> ARLGRQALLFPLCLVLYEFSTYIGNDMIQPGMLAVVEQYQAGIDWVPTSMTAYLAGGMFLQWLLGPLSDRIGRRPVMLAGVVWFIVTCLAILLAQNIEQFTLLRFLQGISLCFIGAVGYAAIQESFEEAVCIKITALMANVALIAPLLGPLVGAAWIHVLPWEGMFVLFAALAAISFFGLQRAMPETATRIGEKLSLKELGRDYKLVLKNGRFVAGALALGFVSLPLLAWTAQSPIIIITGEQLSSYEYGLLQVPIFGALIAGNLLLARLTSRRTVRSLIIMGGWPIMIGLLVAAAATVISSHAYLWMTAGLSIYAFGIGLANAGLVRLTLFASDMSKGTVSAAMEMLQMLIFTVGIEISKHAWLNGGNGLFNLFNLVNGILWLSLMVI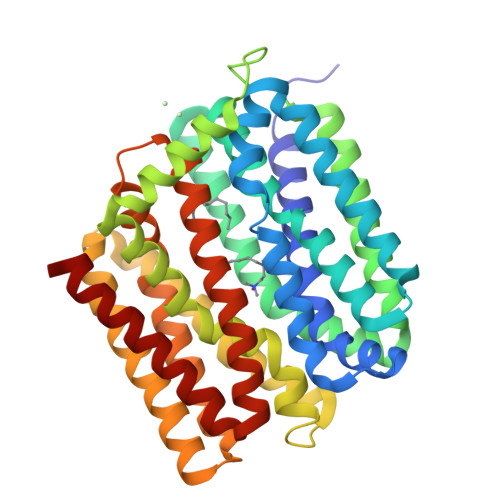FLK>MENTENSVDSKSIKNLEPKIIHGSESMDSGISLDNSYKMDYPEMGLCIIINNKNFHKSTGMTSRSGTDVDAANLRETF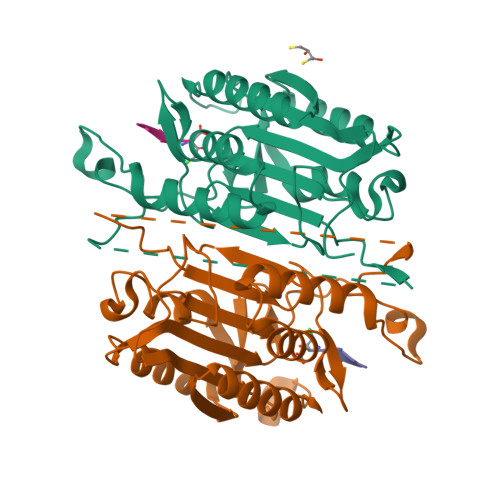RNLKYEVRNKNDLTREEIVELMRDVSKEDHSKRSSFVCVLLSHGEEGIIFGTNGPVDLKKITNFFRGDRCRSLTGKPKLFIIQACRGTELDCGIETDSGVDDDMACHKIPVEADFLYAYSTAPGYYSWRNSKDGSWFIQSLCAMLKQYADKLEFMHILTRVNRKVATEFESFSFDATFHAKKQIPCIDSMLTKELYFYHL[2x]>[6x]SIVTKSIVNADAEARYLSPGELDRIKSFVSSGEKRLRIAQILTDNRERIVKQAGDQLFQKRPDVVSPGGNAYGQEMTATCLRDLDYYLRLITYGIVAGDVTPIEEIGIVGVREMYKSLGTPIDAVAAGVSAMKNVASSILSAEDAAEAGAYFDYVAGALA;>[6x]M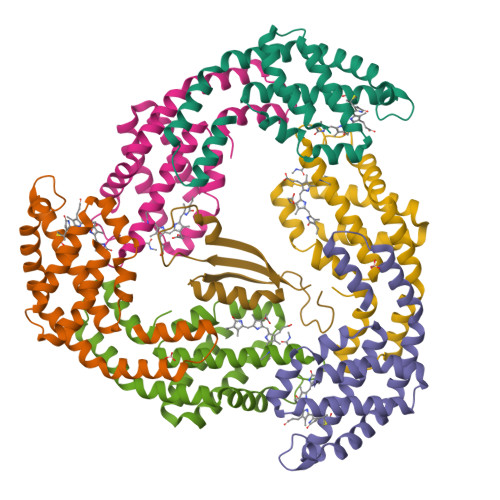QDAITAVINSSDVQGKYLDTAALEKLKSYFSTGELRVRAATTIAANAAAIVKEAVAKSLLYSDITRPGGNMYTTRRYAACIRDLDYYLRYATYAMLAGDPSILDERVLNGLKETYNSLGVPISATVQAIQAMKEVTASLVGPDAGKEMGVYFDYICSGLS;>[2x]GRLFKITACVPSQTRIRTQRELQNTYFTKLVPYENWFREQQRIQKMGGKIVKVELATGKQGINTGLA> GSRISAEGSQACAKGCELCSEVNGCLKCSPKLFILLERNDIRQVGVCLP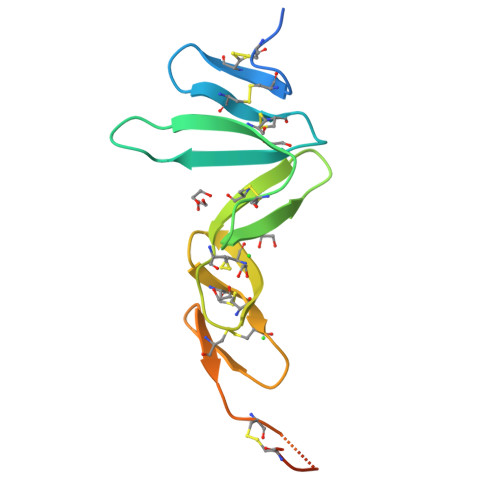SCPPGYFDARNPDMNKCIKCKIEHCEACFSHNFCTKCKEGLYLHKGRCYPACPEGSSAANGTMECSSPAAAHHHHHH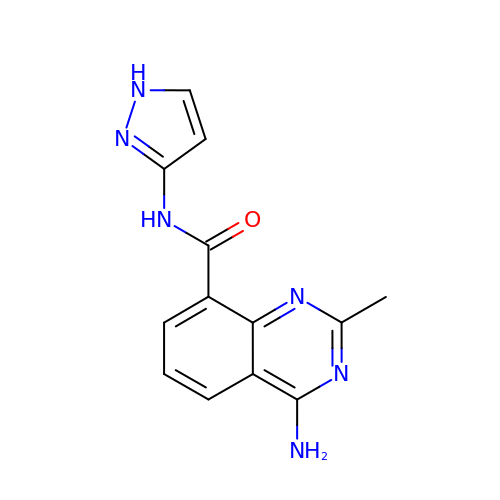4-amino-2-methyl-N-(1H-pyrazol-3-yl)quinazoline-8-carboxamide | C13 H12 N6 O | DMLHUAFVSLGSDJ-UHFFFAOYSA-N CYTIDYL-2'-5'-PHOSPHO-GUANOSINE | C19 H25 N8 O12 P | 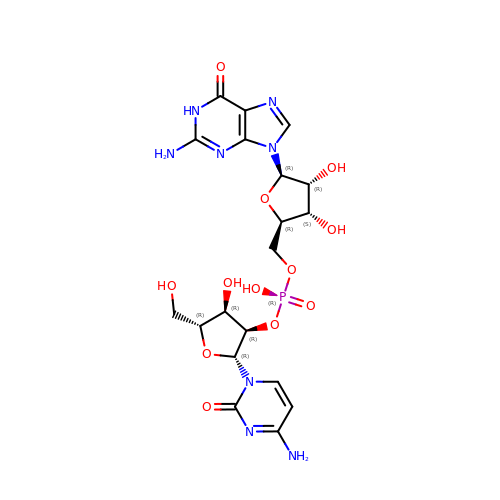QZDUXDLOEVJGDG-VMIOUTBZSA-N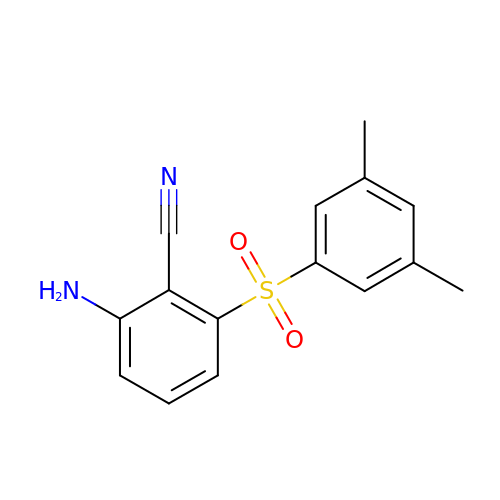2-AMINO-6-(3,5-DIMETHYLPHENYL)SULFONYLBENZONITRILE | C15 H14 N2 O2 S | SWGDXLAZBZDUBR-UHFFFAOYSA-N~{N}-[(4-methoxyphenyl)methyl]-4-(pyridin-4-ylmethyl)aniline | C20 H20 N2 O | 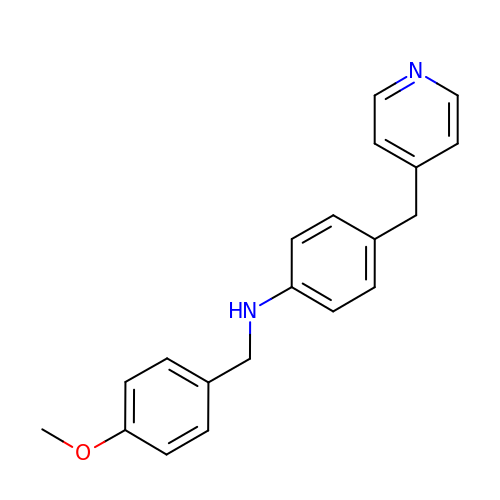FVAKBCRCJCQWCW-UHFFFAOYSA-N> MPAPAADMTTLAGHQQLWDTVMKRRQKREDERIAPPLIRLWDGDYKLRGQLVGERSHKFEFIENETGTASITISLDHYLAKW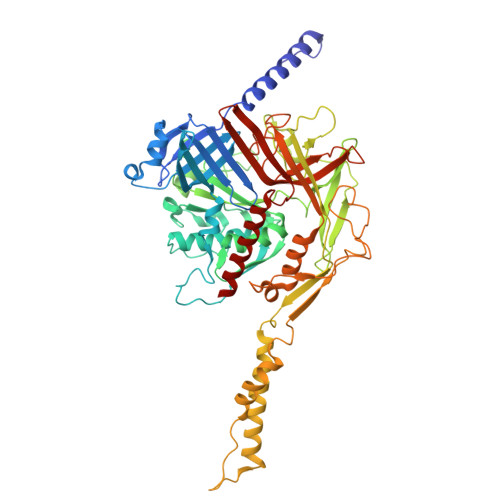IASHKGRARRNVHVSFDKQGARWTGRMDHYDIVRTKEGDVYMEVVFKHDYEELKHIYVWANPFLRPEFQFPKLWVMFGPAKWALLLTLFVNILRLETSLWTLPDNPLDISEWFPFSLNPGNWRNIVKPFPFLADNSPLTIVFSRFKSFHDTAKNVLADSQLTIVCRRYFHGEDPHPFAELSGELGLPLIEGIASLIPLRHGCLVWDIVDNSGWGSETAFGGSLLTGLVRAVMNIASDGMTEGIDIYTGLPTYPGEYYTPGFLGTYPKAPHVVFMESPYTGIESSKFTYTEATDTSFVLGGQSMPGVNEVISAGINMGGDFLTSLINSQLATLGAFGGAIDLPPLGGIMDAVARPLYENVVLAFMEIPTLRAAGLSLPIAGLEDIVTGLGDFHYNEGWVDGADKAFTISAIMAARAKQWATRAKHSHEIQVSDAAPYIIGERGHGHFWLGDRVGTTVLGYPDPYTIFVERVTKLTYEWTSDGPKGWTITIGYKEPEDPILKAFELIQYINSNLGQLGIL>[12x]MGRILDISGQPFDFDDEMQSRSDELAMVMKRTQEHPSSGVTPNRAAQMLRDAERGDLTAQADLAFDMEEKDTHLFSELSKRRLAIQALEWRIAPARDASAQEKKDADMLNEYLHDAAWFEDALFDAGDAILKGYSMQEIEWGWLGKMRVPVALHHRDPALFCANPDNLNELRLRDASYHGLELQPFGWFMHRAKSRTGYVGTNGLVRTLIWPFIFKNYSVRDFAEFLEIYGLPMRVGKYPTGSTNREKATLMQAVMDIGRRAGGIIPMGMTLDFQSAADGQSDPFMAMIGWAEKAISKAILGGTLTTEAGDKGARSLGEVHDEVRREIRNADVGQLARSINRDLIYPLLALNSDSTIDINRLPGIVFDTSEAGDITALSDAIPKLAAGMRIPVSWIQEKLHIPQPVGDEAVFTIQPVVPDNGSQKEAALSAEDIPQEDDIDRMGVSPEDWQRSVDPLLKPVI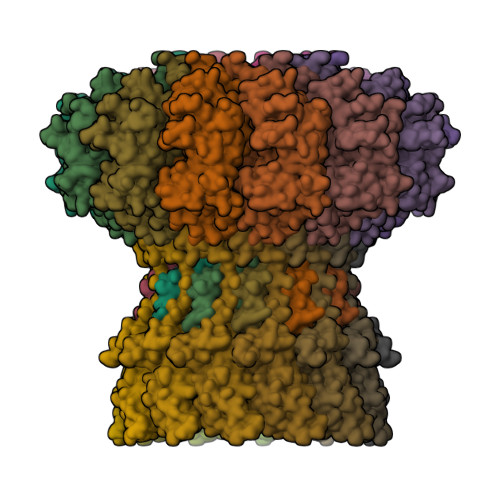FSVLKDGPEAAMNKAASLYPQMDDAELIDMLTRAIFVADIWGRLDAAADH;>[12x]MNYATVNDLCARYTRTRLDILTRPKTADGQPDDAVAEQALADASAFIDGYLAARFVLPLTVVPSLLKRQCCVVAWFYLNESQPTEQITATYRDTVRWLEQVRDGKTDPGVESRTAASPEGEDLVQVQSDPPVFSRKQKGFI>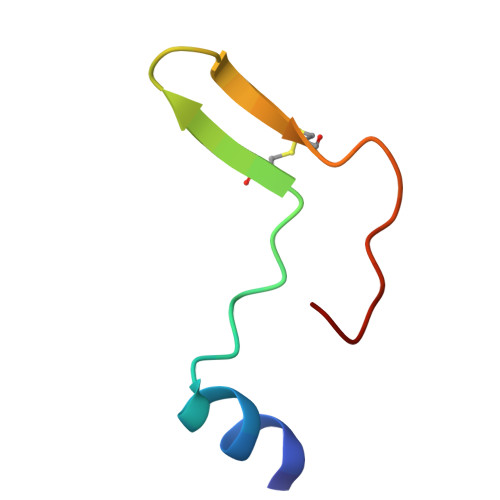 DIVQHMEDIGGAPPVSCVTNEILGVTCAPQAIAKATX DING is a family of proteins with molecular mass of approximately 40 kDa, with a conserved N-terminal sequence of DINGGG. DING proteins are one of three families within a superfamily of bacterial phosphate-binding proteins. To date, the crystal structures of two DING proteins, i.e. human phosphate-binding protein (HPBP) and DING protein from Pseudomonas fluorescens SBW25 (PflDING), have been reported. In both structures, a phosphate ion was captured in a binding cleft between two domains.

In the present study, HPBP with a single mutation was unexpectedly crystallized during a crystallization trial of a certain protein–RNA complex, as was the case for the first crystal of HPBP. We attempted to crystallize a protein complex composed of proteins of 53 kDa, 52 kDa and 11 kDa in complex with its substrate. After crystallization trials and optimization, small crystals were obtained, and a high-resolution X-ray diffraction dataset (1.35 Å resolution) was collected. The crystal belonged to space group C2 with unit-cell parameters a = 94.3 Å, b = 87.1 Å, c = 88.6 Å, β = 90.82°. However, the calculated asymmetric unit (727644 Å3) was too small to locate any of the components. The results of SDS-PAGE of these crystals indicated a protein with a molecular mass of approximately 40 kDa that corresponded to none of the target proteins. To identify the observed protein, it was digested with trypsin and the resultant fragments were analysed by LC-MS. Mascot search of the obtained molecular masses suggested HPBP, a member of the DING protein family, as a candidate. Surprisingly, HPBP (space group C2221, a = 96.3 Å, b = 86.8 Å, c = 89.9 Å) was identified again. Taken together, it is plausible that HPBP was a contaminant in the BSA used for substrate preparation.

>[2x]DINGGGATLPQKLYLTPDVLTAGFAPYIGVGSGKGKIAFLENKYNQFGTDTTKNVHWAGSDSKLTATELATYAADKEPGWGKLIQVPSVATSVAIPFRKAGANAVDLSVKELCGVFSGRIADWSGITGAGRSGPIQVVYRAESSGTTELFTRFLNAKCTTEPGTFAVTTTFANSYSLGLTPLAGAVAATGSDGVMAALNDTTVAEGRITYMSPDFAAPTLAGLDDATKVARVGKGVVNGVAVEGKSPAAANVSAAISVVPLPAAADRGNPDVWVPVFGATTGGGVVAYPDSGYPILGFTNLIFSQCYANATQTGQVRDFFTKHYGTSANNDAAIEANAFVPLPSNWKAAVRASFLTASNALSIGNTNVCNGKGRPQ6-CARBOXYPIPERIDINE | C6 H11 N O2 | 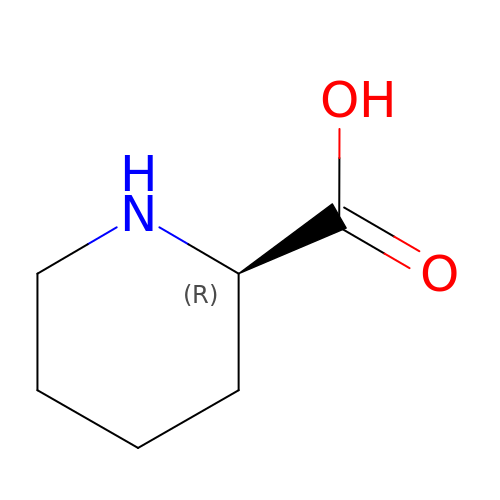HXEACLLIILLPRG-RXMQYKEDSA-N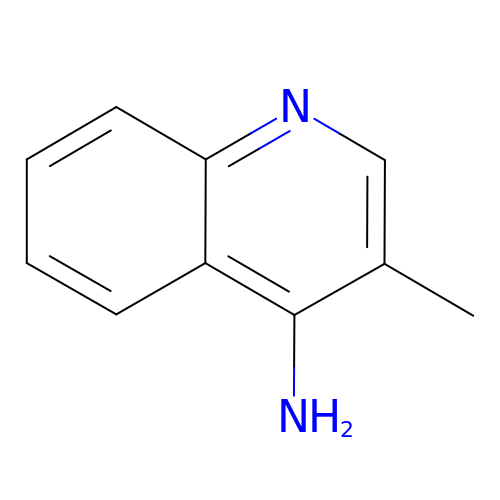3-methylquinolin-4-amine | C10 H10 N2 | LHHFYJQGCWEYNA-UHFFFAOYSA-N> SLEGGVVVPVDYHLLMMFTKAEHNAPLQAKARVALSSLLRLA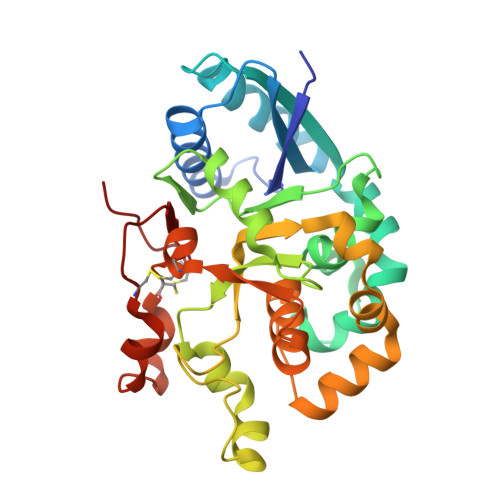KFEAHEVLNLHFVSEEASREVAKALLRELLPPAAGFKCKVIFHDVAVLTDKLFPVVEAMQKYFSAGSGTYYSDSIFFLSVAMHQIMPKEIPRIIQLDLDLKYKTNIRELFEEFDNFLPGAVIGIAREMQPVYRHTFWQFRHENPKTRVGDPPPEGLPGFNSGVMLLNLEAMRQSPLYSHLLEPSWVQQLADKYHFRGHLGDQDFFTMIGMEHPELFHVLDCTWNRQLCTWWRDHGYSDVFQAYFRCEGHVKIYHGNCNTPIPED> SMCKPITGTINDLNQQVWTLQGQNLVAVPRSDSVTPVTVAVITCKYPEALEQGRGDPIYLGIQNPEMCLYCEKVGEQPTLQLKEQKIMDLYGQPEPVKPFLFYRAKTGRTSTLESVAFPDWFIASSKRDQPIILTSELGKSYNTAFELNIND

IL-36 family cytokines, which are members of the larger IL-1R superfamily, include three agonists (IL-36α, IL-36β, and IL-36γ) and an antagonist, IL-36Ra. All three agonists bind to and signal through a heterodimeric receptor composed of IL-36 receptor subunit (IL-36R), which binds selectively to all IL-36 family members and an IL-1RAcP co-receptor subunit, which is shared with several other IL-1R superfamily members including IL-1β. Binding of IL-36 agonists to IL-36R/IL-1RAcP heterodimer induces signaling through MyD88/IRAK complex leading to the activation of NF-κB and MAPKs signaling cascades shared among IL-1R superfamily members.

The co-crystal structure of human IL-36γ and A-552 was determined to 2.0 Å resolution. In the new IL-36γ structure, A-552 is bound at the center of the cytokine’s β-trefoil fold with a calculated pocket volume of 150 Å3. When comparing the apo and ligand bound structures, the C-terminal tail moves in order to open the pocket for ligand binding. Firstly, the carboxylate at the center of the ligand makes key hydrogen bond interactions to residues Arg121 and Lys123. Arg121 also provides a π-cation stacking interaction to the central ligand pyrimidine ring. Additionally, the methyl aniline inserts into the back of the ligand pocket in a hydrophobic space which is outlined by residues Val58, Leu130, Leu165 and Ile27. The structure demonstrates why A-552 likely has a higher affinity than A-553 as A-552 presents the carboxylate in an optimal orientation to engage basic residues Arg121 and Lys123 with respect to the flanking phenyl rings. In this binding pose, less active enantiomer A-553 would not be able to make the necessary hydrogen bonds to these residues due to lack of proximity. This x-ray structure also rationalizes why A-552 does not show affinity for either mouse IL-36γ, human IL-36α or IL-36β. The terminal biphenyl group does not play any specific role in the ligand binding to IL-36γ; however, it projects into the space where IL-36R would be in the IL-36γ/IL-36R/IL-1RAcP ternary complex. The trajectory of the terminal biphenyl group can sterically occlude the IL-36R linker (connecting the D3 and D1/D2 domains) from binding to IL-36γ ligand.> SHMTAVTLDGGWRVRLVPGQEQGKTYPKAAAWLPAQVPGAVQTDLIAAKIVPDPFYRDNEGKIQWAGLSDWQYQTRFTVDAATLKREHVELVFDGLDTFAEVTLNGKQLLSADNMFRQWRVDAKSLLKRGDNLLEVKLYSPIKKIQPWLAKQPYALPGAYDSAFGDEPEARHSSTYVRKAPYNFGWDWGPRMVNAGIWKDVRVEAWDAVRVDGLHIAQQRVDAHSAQVQAQLDLQAGRSGPVQVTLDVLGPDGQKVGQFTQDAVVDPGQNRVDLAVRIANPKRWFPAGYGAQDRYTFVASVRDADGDSQQIKRVTGLRSVELRREKDRFGKSMEIVINGIPIFAKGANLIPLDAFPARVTHERMRSTLQDARDANMNMLRMWGGGHYQDDYFYDVADELGIMI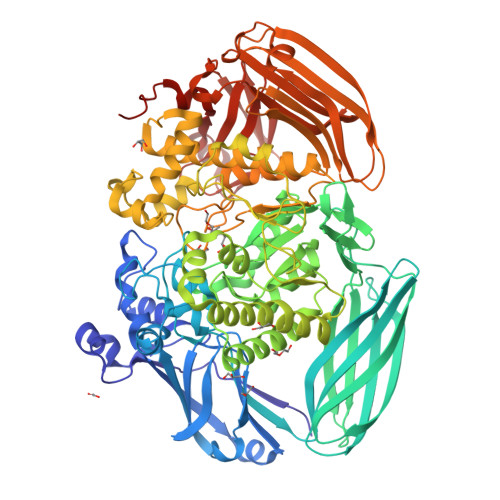WQDFMFGGAVPPYDVEFRENTRQEAIEQVKRLRDHPSLVLWCGNNEVQTGWENWGDRVKFKQSVDPEERTRIERGMTTLFGTVFREVVATYDSDVPYWATSPGTDFDGAADQTNDGDMHYWKVWGGPALPVTEYLNVTPRFMSEYGLQSFPDMRTVRAFAEPGDMDPESPVMRVHQKFDKGNGNKRLMLYIRREFGEPKDFESFVYLSQLMQAEGINIAASHLRASRPQSMGSLYWQLNDVWPGASWSSVDYYGRWKALHYHARRFYAPEMIAALRNDKGQTEVSLVSDRTTPLTARWRMRVMGMDGKVLSKREEKASVNALSSQHVGNFSDKQLLGSADPKRTYAVFELLDGDTLLSREVVFFAPAKQLALPAAKIDSQWRADGDGYALTLTSDTLAREVWLSFGDVDATLSDNAFDLLPGEPLTVRVTSKAALAQLQSALQVRDLAATLAGAPPEPQ>HPSSPPVVDTVHGKVLGKFVSLEGFAQPVAIFLGIPFAKPPLGPLRFTPPQPAEPWSFVKNATSYPPMCTQDPKAGQLLSELFTNRKENIPLKLSEDCLYLNIYTPADLTKKNRLPVMVWIHGGGLMVGAASTYDGLALAAHENVVVVTIQYRLGIWGFFSTGDEHSRGNWGHLDQVAALRWVQDNIASFGGNPGSVTIFGESAGGESVSVLVLSPLAKNLFHRAISESGVALTSVLVKKGDVKPLAEQIAITAGCKTTTSAVMVHCLRQKTEEELLETTLKMKFLSLDLQGDPRESQPLLGTVIDGMLLLKTPEELQAERNFHTVPYMVGINKQEFGWLIPMLMSYPLSEGQLDQKTAMSLLWKSYPLVCIAKELIPEATEKYLGGTDDTVKKKDLFLDLIADVMFGVPSVIVARNHRDAGAPTYMYEFQYRPSFSSDMKPKTVIGDHGDELFSVFGAPFLKEGASEEEIRLSKMVMKFWANFARNG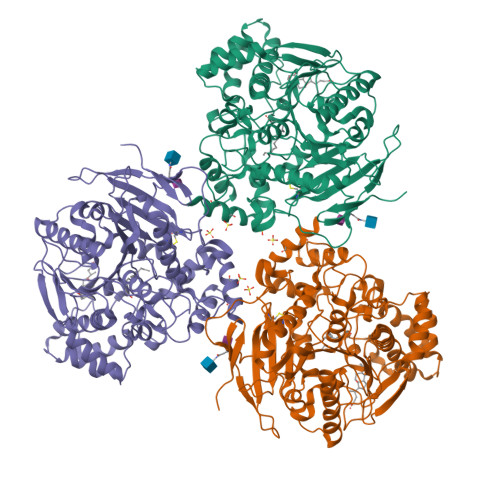NPNGEGLPHWPEYNQKEGYLQIGANTQAAQKLKDKEVAFWTNLFAKKAVEKPPQ[3x]> UUCUGCUG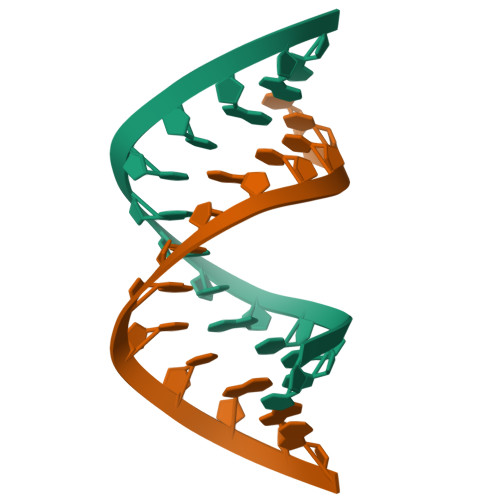CUGAA;> UUCUGCAGCUGAA methyl 6-[6-amino-2-(methylamino)-8-oxo-7,8-dihydro-1H-imidazo[4,5-g]quinazolin-4-yl]-5,6-dideoxy-2-O-methyl-beta-D-ribo-hexofuranoside 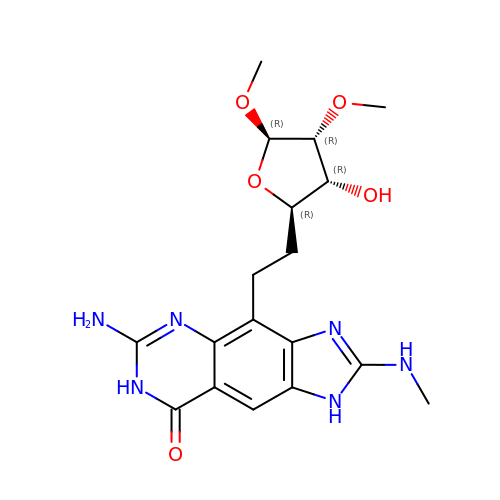| C18 H24 N6 O5 | XTZFREKGNSFRGQ-DSPGLSBSSA-N>[2x]MTKIFAYAIREDEKPFLKEWEDAHKDVEVEYTDKLLTPETVALAKGADGVVVYQQLDYIAETLQALADNGITKMSLRNVGVDNIDMAKAKELGFQITNVPVYSPNAIAEHAAIQAARILRQDKAMDEKVARHDLRWAPTIGREVRDQVVGVVGTGHIGQVFMQIMEGFGAKVITYDIFRNPELEKKGYYVDS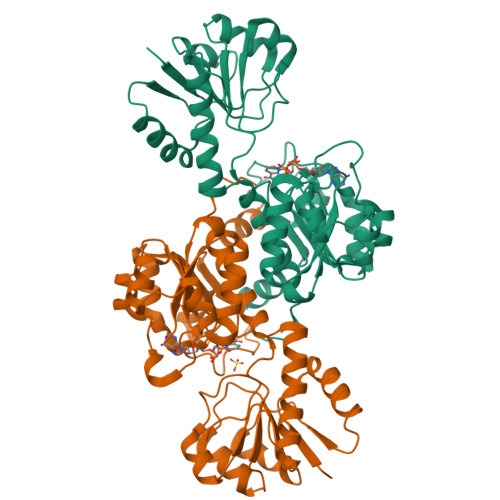LDDLYKQADVISLHVPDVPANVHMINDESIAKMKQDVVIVNVSRGPLVDTDAVIRGLDSGKIFGYAMDVYEGEVGIFNEDWEGKEFPDARLADLIARPNVLVTPHTAFYTTHAVRNMVVKAFDNNLELVEGKEAETPVKVG>MSESQTLDKVYQMKSKPRGYCLIINNHNFAKAREKVPKLHSIRDRNGTH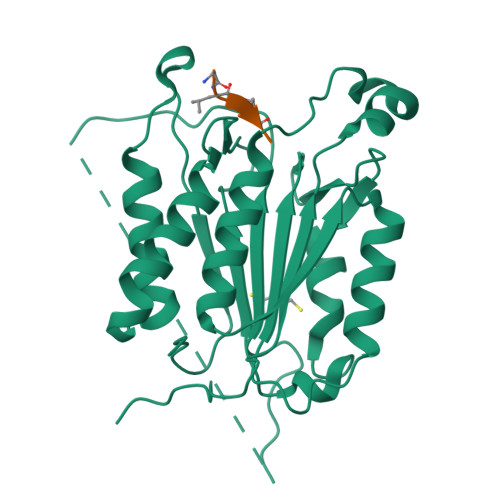LDAGALTTTFEELHFEIKPHDDCTVEQIYEILKIYQLMDHSNMDCFICCILSHGDKGIIYGTDGQEAPIYELTSQFTGLKCPSLAGKPKVFFIQACQGDNYQKGIPVETDSEEQPYLEMDLSSPQTRYIPDEADFLLGMATVNNCVSYRNPAEGTWYIQSLCQSLRERCPRGDDILTILTEVNYEVSNKDDKKNMGKQMPQPTFTLRKKLVFPSDAAALEHHHHHH[4x]> MLADGFETDIAIPSGISRPDAAALQRCEGRVVFLPTIRRQLTLADVAHESFVSGGVSPDTLGLLLAYRRRFPAVITRVLPTRIVACPLDVGLTHAGTVNLRNTSPVDLCNGDPISLVPPVFEGQATDVRLDSLDLTLRFPVPLPSPLAREIVARLVARGIRDLNPSPRNPGGLPDLNVLYYNGSRLSLLADVQQLGPVNAELRSLVLNMVYSITEGTTIILTLIPRLFALSAQDGYVNALLQMQSVTREAAQLIHPEAPALMQDGERRLPLYEALVAWLTHA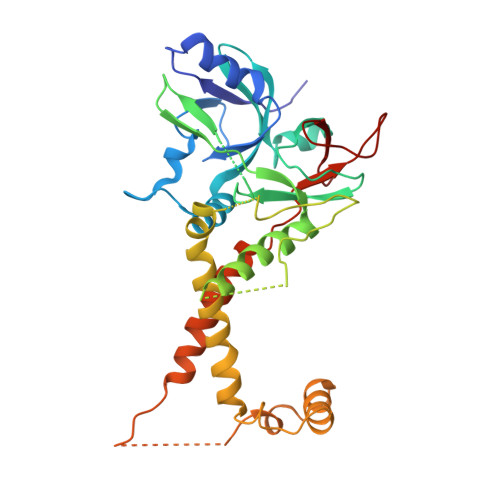GQLGDTLALAPVVRVCTFDGAAVVRSGDMAPVIRYP> MRSRILAIVFAARHVAALPLAAEDAAATLSLTSSASSTTVLPSPTQYTLPNNDPNQGARNASIARKRELFLYGPSTLGQTTFYPTGELGNNISARDVLLWRQDAANQTATAYREANETFADITSRGGFKTLDDFALLYNGHWKESVPEGISKGMLSNCTSDLLFSMERLSSNPYVLKRLHPTKDKLPFSVESKVVKKLTATTLEALHKGGRLFLVDHSYQKKYTPQPGRYAAACQGLFYLDARSNQFLPLAIKTNVGVDLTYTPLDDKDDWLLAKIMFNNNDLFYSQMYHVLFHTIPEIVHEAAFRTLSDRHPVMGVLNRLMYQAYAIRPVGGAVLFNPGGFWDQNFGLPASAAIDFP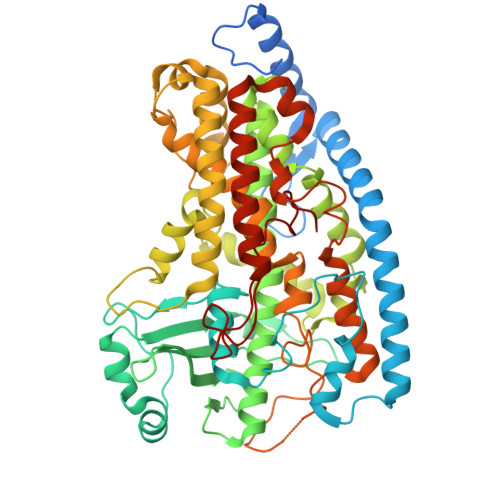GSVYAQGGGGFQAGYLEKDLRSRGLIGEDSGPRLPHFPFYEDAHRLIGAIRRFMQAFVDSTYGADDGDDGALLRDYELQNWIAEANGPAQVRDFPAAPLRRRAQLVDVLTHVAWITGGAHHVMNQGSPVKFSGVLPLHPAALYAPIPTAKGATGNGTRAGLLAWLPNERQAVEQVSLLARFNRAQVGDRKQTVRDAFAAPDLLAGNGPGYAAANARFVEDTGRISREIAGRGFDGKGLSQGMPFVWTALNPAVNPFFLSV>[2x]MHHHHHHSMGKRNKPGKATGKGKPVNNKWLNNAGKDLGSPVPDRIANKLRDKEFKSFDDFRKKFWEEVSKDPELSKQFSRNNNDRMKVGKAPKTRTQDVSGK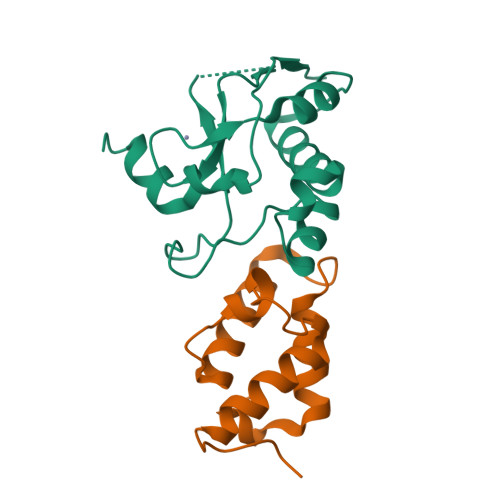RTSFELHAEKPISQNGGVYDMDNISVVTPKRHIDIHRGK;>MELKHSISDYTEAEFLQLVATICDADATSEEELDKLITHFGEMTEHPSGSDLIYYPEEGDDDSPSGIVNTVKQWRAANGKSGFKQG[2x]> ALEEAPWPPPEGAFVGFVLSRKEPMWADLLALAAARGGRVHRAPEPYKALRDLKEERGLLAKDLSVLALREGLGLPPGDDPMLLAYLLDPSNTTPEGVARRYGGEWTEEAGERAALSERLFANLWGRLEGEERLLWLYREVERPLSAVLAHMEATGVRLDVAYLRALSLEVAEEIARLEAEVFRLAGHPFNLNSRDQLERVLFDELGLPAIGKTEKTGKRSTSAAVLEALREAHPIVEKILQYRELTKLKSTYIDPLPDLIHPRTGRL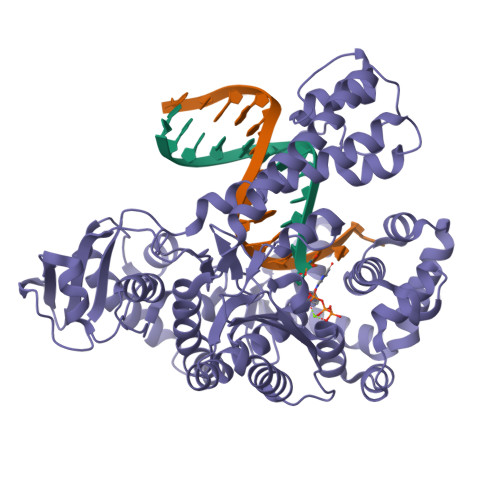HTRFNQTATATGRLSSSDPNLQNIPVRTPLGQRIRRAFIAEEGWLLVALDYSQIELRVLAHLSGDENLIRVFQEGRDIHTETASWMFGVPREAVDPLMRRAAKTINFGVLYGMSAHRLSQELAIPYEEAQAFIERYFQSFPKVRAWIEKTLEEGRRRGYVETLFGRRRYVPDLEARVKSVREAAERMAFNMPVQGTAADLMKLAMVKLFPRLEEMGARMLLQVHDELVLEAPKERAEAVARLAKEVMEGVYPLAVPLEVEVGIGEDWLSAK> CGTAC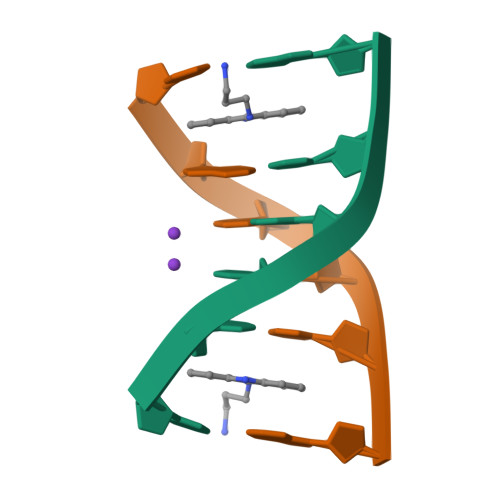G>[2x]QVTTEAPAKVVKHSKKQDENIVVNKFKPKEPYVGRCLLNTKITGDDAPG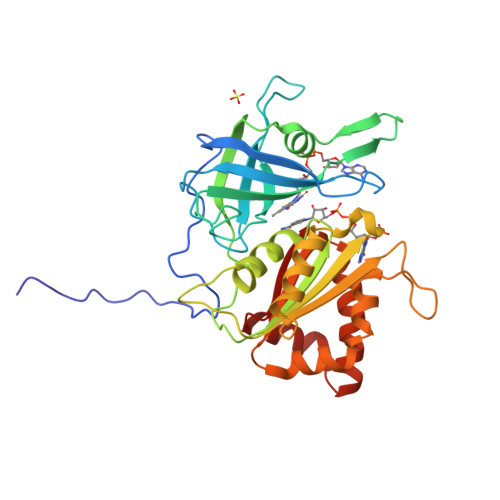ETWHMVFSTEGEVPYREGQSIGIVPDGIDKNGKPHKLRLYSIASSAIGDFGDSKTVSLCVKRLVYTNDAGEVVKGVCSNFLCDLKPGSEVKITGPVGKEMLMPKDPNATVIMLGTGTGIAPFRSFLWKMFFEKHEDYQFNGLAWLFLGVPTSSSLLYKEEFEKMKEKAPENFRLDFAVSREQVNDKGEKMYIQTRMAQYAEELWELLKKDNTFVYMCGLKGMEKGIDDIMVSLAAKDGIDWIEYKRTLKKAEQWNVEVS> GAEFKGLRVDMFLYNLTLQRATGISFAIHGNFSGTKQQEIVVSRGKILELLRPDPNTGKVHTLLTVEVFGVIRSLMAFRLTGGTKDYIVVGSDSGRIVILEYQPSKNMFEKIHQETFGKSGCRRIVPGQFLAVDPKGRAVMISAIEKQKLVYILNRDAAARLTISSPLEAHKANTLVYHVVGVDVGFENPMFACLEMDYEEADNDPTGEAAANTQQTLTFYE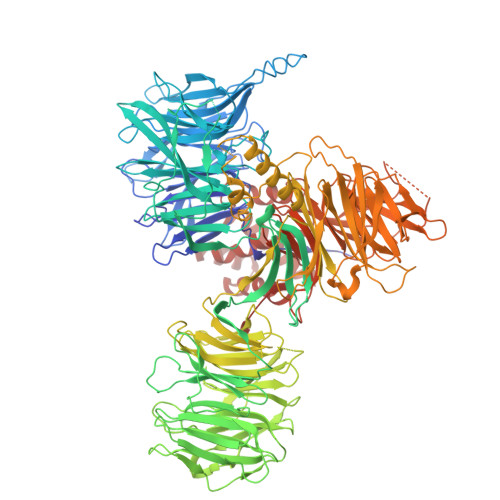LDLGLNHVVRKYSEPLEEHGNFLITVPGGSDGPSGVLICSENYITYKNFGDQPDIRCPIPRRRNDLDDPERGMIFVCSATHKTKSMFFFLAQTEQGDIFKITLETDEDMVTEIRLKYFDTVPVAAAMCVLKTGFLFVASEFGNHYLYQIAHLGDDDEEPEFSSAMPLEEGDTFFFQPRPLKNLVLVDELDSLSPILFCQIADLANEDTPQLYVACGRGPRSSLRVLRHGLEVSEMAVSELPGNPNAVWTVRRHIEDEFDAYIIVSFVNATLVLSIGETVEEVTDSGFLGTTPTLSCSLLGDDALVQVYPDGIRHIRADKRVNEWKTPGKKTIVKCAVNQRQVVIALTGGELVYFEMDPSGQLNEYTERKEMSADVVCMSLANVPPGEQRSRFLAVGLVDNTVRIISLDPSDCLQPLSMQALPAQPESLCIVEMGGTEKQDELGERGSIGFLYLNIGLQNGVLLRTVLDPVTGDLSDTRTRYLGSRPVKLFRVRMQGQEAVLAMSSRSWLSYSYQSRFHLTPLSYETLEFASGFASEQCPEGIVAISTNTLRILALEKLGAVFNQVAFPLQYTPRKFVIHPESNNLIIIETDHNAYTEATKAQRKQQMAEEMVEAAGEDERELAAEMAAAFLNENLPESIFGAPKAGNGQWASVIRVMNPIQGNTLDLVQLEQNEAAFSVAVCRFSNTGEDWYVLVGVAKDLILNPRSVAGGFVYTYKLVNNGEKLEFLHKTPVEEVPAAIAPFQGRVLIGVGKLLRVYDLGKKKLLRKCENKHIANYISGIQTIGHRVIVSDVQESFIWVRYKRNENQLIIFADDTYPRWVTTASLLDYDTVAGADKFGNICVVRLPPNTNDEVDEDPTGNKALWDRGLLNGASQKAEVIMNYHVGETVLSLQKTTLIPGGSESLVYTTLSGGIGILVPFTSHEDHDFFQHVEMHLRSEHPPLCGRDHLSFRSYYFPVKNVIDGDLCEQFNSMEPNKQKNVSEELDRTPPEVSKKLEDIRTRYAFDYKDDDDK> MLAGLVPAPDHGMREEILGDRSRLIRQR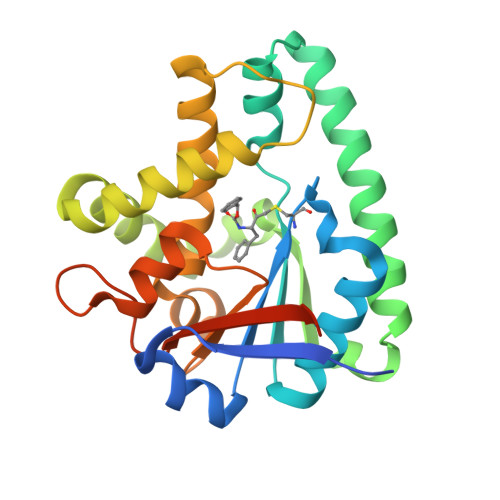GEHALIGICAGNSYFSQKNTVMLLQWAGQRFERTDVVYVDTHIDEMLIADGRSAQEAERSVKRTLKDLRRRLRRSLESVGDHAERFRVRSLSELQETPEYRAVRERTDRAFEEDAEFATACEDMVRAVVMNRPGDGVGISAEHLRAGLNYVLAEAPLFADSPGVFSVPSSVLCYHIDTPITAFLSRRETGFRAAEGQAYVVVRPQELADAARSHHHHHH>MAEAASCARKGTKYAEGTQPFTVLIEGNIGSGKTTYLNHFEKYKNDICLLTEPVEKWRNVNGVNLLELMYKDPKKWAMPFQSYVTLTMLQSHTAPTNKKLKIMERSIFSARYCFVENMRRNGSLEQGMYNTLEEWYKFIEESIHVQADLIIYLRTSPEVAYERIRQRARSEESCVPLKYLQELHELHEDWLIHQRRPQSCKVLVLDADLNLENIGTEYQRSESSIFDAISSNQQP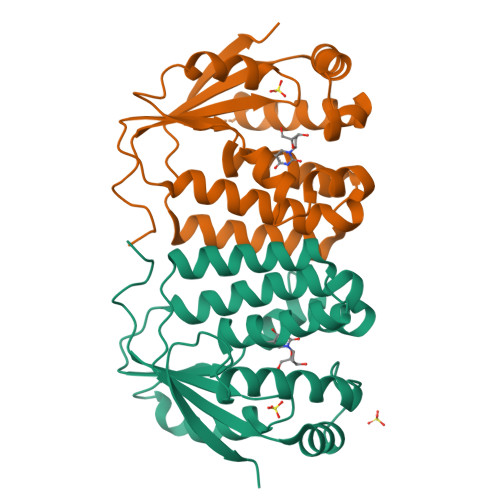SPVLVSPSKRQRVAR[8x]(2R)-2-[(1-aminoisoquinolin-6-yl)amino]-4,11-diazatricyclo[14.2.2.1~6,10~]henicosa-1(18),6(21),7,9,16,19-hexaene-3,12-dione 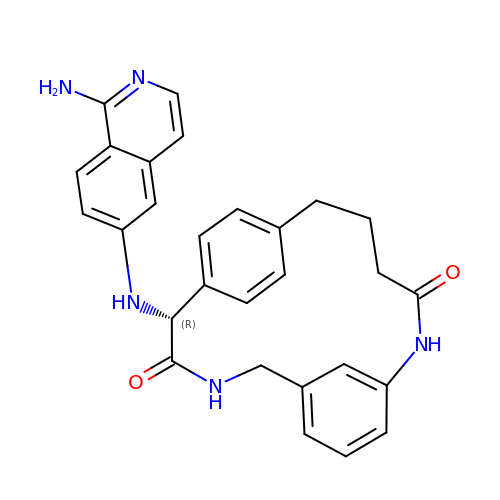| C28 H27 N5 O2 | LXFPTSIBSQOGTO-AREMUKBSSA-N> MASMTGGQQMGRGSMIFSVDKVRADFPVLSREVNGLPLAYLDSAASAQKPSQVIDAEAEFYRHGYAAVHRGIHTLSAQATEKMENVRKRASLFINARSAEELVFVAGTTEGINLVANSWGNSNVRAGDNIIISQMEHHANIVPWQMLCARVGAELRVIPLNPDGTLQLETLPTLFDEKTRLLAITHVSNVLGTENPLAEMITLAHQHGAKVLVDGAQAVMHHPVDVQALDCDFYVFSGHKLYGPTGIGILYVKEALLQEMPPWEGGGSMIATVSLSEGTTWTKAPWRFEAGTPNTGGIIGLGAALEYVSALGLNNIAEYEQNLMHYALSQLESVPDLTLYGPQNRLGVIAFNLGKHHAYDVGSFLDNYGIAVRTGHHCAMPLMAYYNVPAMCRASLAMYNTHEEVDRLVTGLQRIHR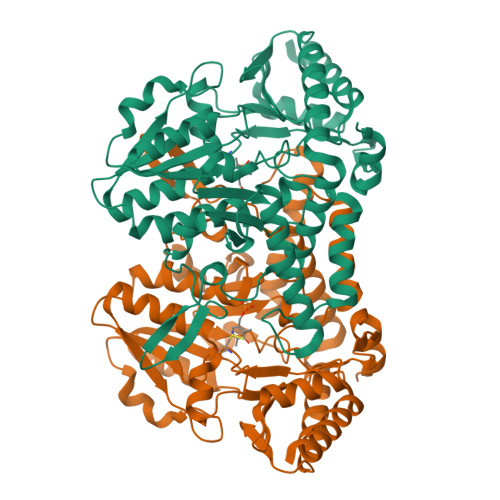LLG> SKKISDHTEAEFFSLISELFNRSFSSEKERDVVVYAIVNAAQHPDGTDIIFYPKEDEEDSPEGVLKRIKEWRAANGL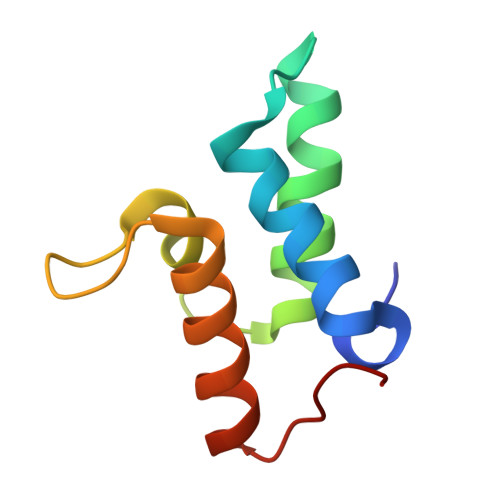PGFKA>SMSKRTFSTVLPQIDTTGQLFVQTRKGQEVLIKVKHFMKQHILPAEKEVTEFYVQNENSVDKWGKPLVIDKLKEMAKVEGLWNLFLPAVSGLSHVDYALIAEETGKCFFAPDVFNCQAPDTGNMEVLHLYGSEEQKKQWLEPLLQGNITSCFCMTEPDVASSDATNIECSIQRDEDSYVINGKKWWSSGAGNPKCKIAIVLGRTQNTSLSRHKQHSMILVPMNTPGVKIIRPLSVFGYTDNFHGGHFEIHFNQVRVPATNLILGEGRGFEISQGRLGPGRIHHCMRTVGLAERALQIMCERATQRIAFKKKLYAHEVVAHWIAESRIAIEKIRLLTLKAAHSMDTLGSAGAKKEIAMIKVAAPRAVSKIVDWAIQVCGGAGVSQDYPLANMYAITRVLRLADGPDEVHLSAIATMELRD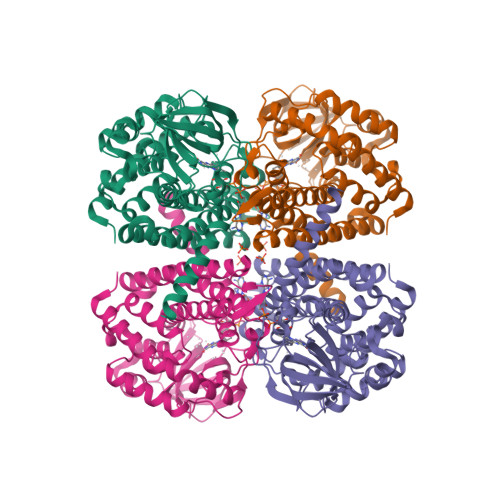QAKRLTAKI[2x]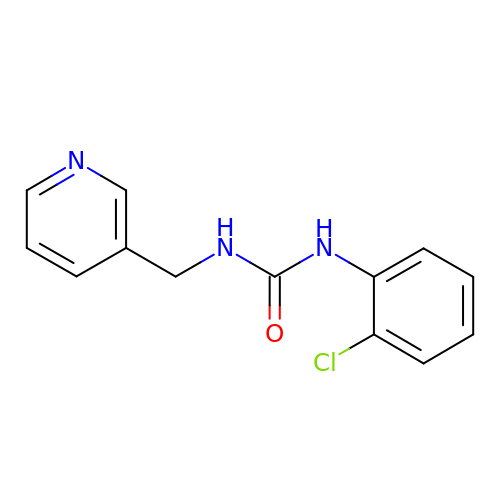1-(2-chlorophenyl)-3-(pyridin-3-ylmethyl)urea | C13 H12 Cl N3 O | BYPMLXJTXCLBOI-UHFFFAOYSA-N>[2x]MASVVGTPKSAEQIQQEWDTNPRWKDVTRTYSAEDVVALQGSVVEEHTLARRGAEVLWEQLHDLEWVNALGALTGNMAVQQVRAGLKAIYLSGWQVAGDANLSGHTYPDQSLYPANSVPQVVRRINNALQRADQIAKIEGDTSVENWLAPIVADGEAGFGGALNVYELQKALIAAGVAGSHWEDQLASEKKCGHLGGKVL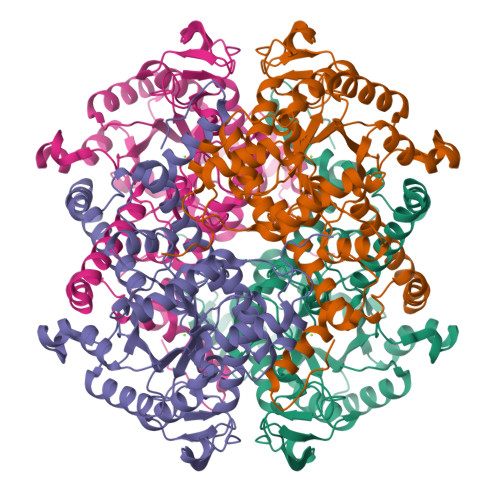IPTQQHIRTLTSARLAADVADVPTVVIARTDAEAATLITSDVDERDQPFITGERTREGFYRTKNGIEPCIARAKAYAPFADLIWMETGTPDLEAARQFSEAVKAEYPDQMLAYNCSPSFNWKKHLDDATIAKFQKELAAMGFKFQFITLAGFHALNYSMFDLAYGYAQNQMSAYVELQEREFAAEERGYTATKHQREVGAGYFDRIATTVDPNSSTTALTGSTEEGQFH> X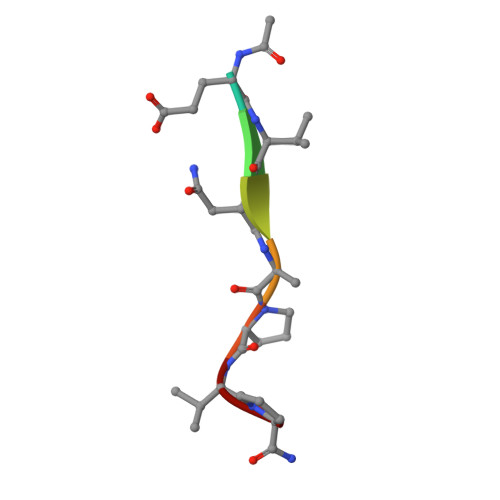EVNAPVP> GSSMASANLEGDALHTLRVTLVDPNNVLQSWDPTLVNPCTWFHVTCNNENSVIRVDLGNAELSGHLVPELGVLKNLQYLELYSNNITGPIPSNLGNLTNLVSLDLYLNSFSGPIPESLGKLSKLRFLRLNNNSLTGSIPMSLTNITTLQVLDLSNNRLSGSV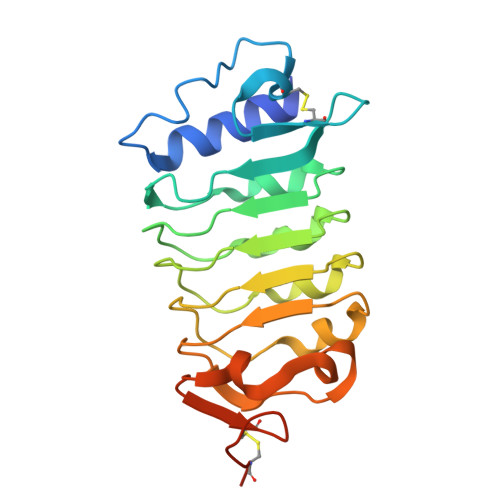PDNGSFSLFTPISFANNLDLCGPVTSHPCPGSLENLYFQGA> DDYSFSCYSQLEVNGSQHSLTCAFEDPDVNITNLEFEICGALVEVKCLN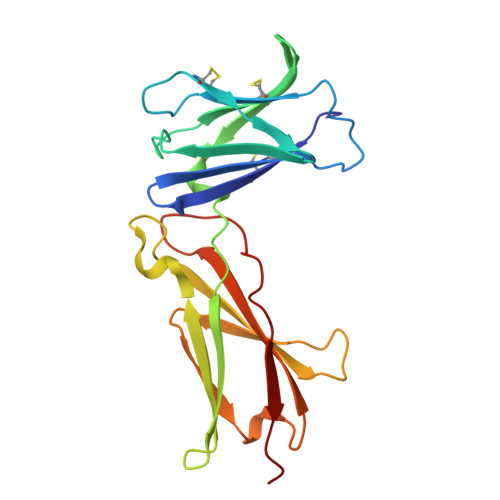FRKLQEIYFIETKKFLLIGKSNICVKVGEKSLTCKKIDLTTIVKPEAPFDLSVVYREGANDFVVTFNTSHLQKKYVKVLMHDVAYRQEKDENKWTHVNLSSTKLTLLQRKLQPAAMYEIKVRSIPDHYFKGFWSEWSPSYYFRTPEI> MNEFVEDHRSECQIGNIPSSVNNAKLPDPFMGLDGKRISSKADWKCRREEIGAMYEKLMFGTKPRNPEKVEGSYSGGKLTIKVTDKGKSGSFSVKISNAGTKDKPKPAMIGFGGGMMGGCGSLGNATNGLDIAQITFNPDDVAPESGGGMFFQLYNQGQGTIIAWAWGVSRIIDALEKTPEAGIDVKHLAMTGCSRWGKGTLAVGAFDERIALTIPQESGSGGASLWRVGAQVNKQKGKQFVQGLSSAGTEGKWMISSFKNYDGKENTLPFDQHMLVAMVAPRALLILDNAGQEWLGEVPSNYCGQASKEVYDALGATENYTYSQEGGHGHCQLPNGQFDEVKDFMNKFLLGKDAKTGKIDYTKNTQTINFKKSEWIDWETPSLKDPAFLYKPAFLYKVVIMHHHHHH

Glucuronoyl esterases (GEs) within the carbohydrate esterase family 15 (CE15) esterase family, in a range of aerobic and anaerobic fungi and bacteria, have been identified as playing an important role in breaking down LCCs by cleaving the ester bond between 4-O-methyl-d-glucuronyl in xylan and alcohol groups in lignin. GEs share an invariant Ser-His-Glu/Asp catalytic triad and employ a conserved catalytic mechanism that involves the formation of an acyl-enzyme covalent intermediate, which is subsequently cleaved through acid-base hydrolysis. Rumen GEs adopt a canonical α/β hydrolase fold: FsCE15, PrCE15, and RfCE15 adopted the canonical α/β-hydrolase fold that is seen in all of the GE structures solved to date. The fold of all three enzymes consists of a central twisted 10 stranded mixed β-sheet flanked by α-helices on either side.

Crystals of FsCE15 belonged to space group P41212 with a single protein molecule in the asymmetric unit. The structure of FsCE15 was refined to Rwork/Rfree of 22.8%/28.5% (respectively) using data to a maximum resolution of 1.93 Å. The putative catalytic nucleophile, general base, and general acid of FsCE15 are Ser346, His482, and Glu369, respectively. The catalytic residues of FsCE15 and PrCE15 are positioned in the canonical conformation characteristic of CE15-B subfamily with the general acid located on a loop at the end of β7. FsCE15 and PrCE15 have a conserved disulfide bond between residues Cys345 - Cys483 and Cys225 - Cys356, respectively, which anchors the general base within optimal hydrogen bonding distance (2.7 Å) to the catalytic serine. Similarly, the addition of a reducing agent lowered the Tm of FsCE15 by 11.5 °C. These results demonstrates the important role that the disulfide bond in the active site of CE15-B GEs plays in stabilizing tertiary structure. FsCE15 has a broad pH profile with maximal activity at pH 8.0. Interestingly, HGT events between Fibrobacterota and AGF were one of the most commonly observed events by Murphey at al.. This observation is supported by our phylogenetic analysis showing that FsCE15 clustered closely with Neocallimastigomycota carbohydrate esterase family 15 esterases. FsCE15 also possesses structural features that are typically observed in fungal GEs including: a shallow active site lacking any of the insertions in the Reg1-Reg3 regions, catalytic residues that adopt a canonical CE15-A active site conformation, and a conserved disulfide bond in the active site. FsCE15 is therefore unique amongst bacterial GEs characterized to date and may represent an intermediate between fungal and bacterial GEs.> GSHMLITASSSKEYLPDLLLFWQNYEYWITNIGLYKTKQRDLTRTPANLDTDTEECMFWMNYLQKDQSFQLMNFAMENLGALYFGSIGDISELYLRVEQYWDRRADKNHSVDGKYWDALIWSVFTMCIYYMPVEKLAEIFSVYPLHEYLGSNKRLNWEDGMQLVMCQNFARCSLFQLKQCDFMAHPDIRLVQAYLILATTTFPYDEPLLANSLLTQCIHTFKNFHVDDFRPLLNDDPVESIAKVTLGRIFYRLCGCDYLQSGPRKPIALHTEV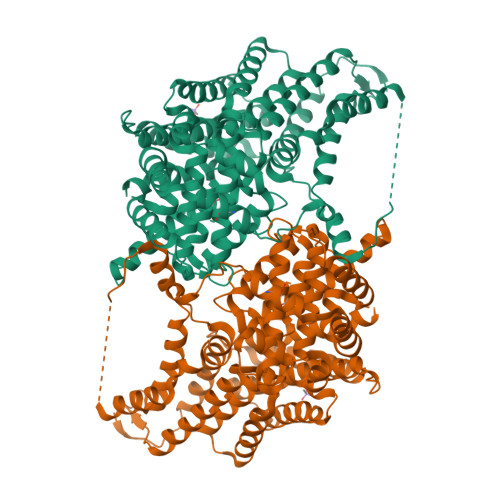SSLLQHAAYLQDLPNVDVYREENSTEVLYWKIISLDRDLDQYLNKSSKPPLKTLDAIRRELDIFQYKVDSLEEDFRSNNSRFQKFIALFQISTVSWKLFKMYLIYYDTADSLLKVIHYSKVIISLIVNNFHAKSEFFNRHPMVMQTITRVVSFISFYQIFVESAAVKQLLVDLTELTANLPTIFGSKLDKLVYLTERLSKLKLLWDKVQLLDSGDSFYHPVFKILQNDIKIIELKNDEMFSLIKGLGSLVPLNKLRQESLLEEEDENNTEPSDFRTIVEEFQSEYNISDILS Sobemoviruses encode serine-like 3C proteases (Pro) that participate in the processing and maturation of other virus-encoded proteins. Its cis and trans activity is mediated by the naturally unfolded virus-genome-linked protein (VPg). Here, we solved a full Pro–VPg 3D structure of ryegrass mottle virus (RGMoV) that demonstrates the structural changes in three different conformations due to VPg interaction with Pro. The overall fold change of Δ117Pro is typical for CLP and is very similar to the structure of SeMV Pro.

We crystallized and solved 3D crystal structures for two catalytically active forms of Δ117Pro: one in its VPg-free form, the second in its VPg-bound state with fused VPg at the C-terminal part (Δ117Pro-E/A-VPg), and one catalytically defective Δ117Procm form with S159/A mutation. First, in the absence of VPg, L87 shifted towards the VPg-binding pocket. In Δ117Pro chain A, it is rotated away from the catalytic triad H49, thereby disrupting the functionality of the catalytic triad since D92 is too far from H49 to ensure any proton transfer. There are several more conformational shifts unique only to Δ117Pro and that are not present in Δ117Procm and Δ117Pro-E/A-VPg. These are the partial unwinding of the βII barrel and subsequent movement of the bII and cII β-strands and the cII/dII loop, and the disordering of the eII/fII loop. While H173 and N183 did not change their positions significantly, H150 and T154 were noticeably shifted due to the movement of bII-cII strands. This shift could also render the Glu-binding site unsuitable for cleavage site recognition.

>AVANSIVSSVAPGKEPGSLVCIQAKDGKVIGMGARVHCGPATVLVTAGHVLKKGMIADLYLAKYSVSSKEGKRVLMDPTWKIEYGSLNKEADVISVQVPAAVWSRLGVTAARVRKPTVKVPVLAYGGEASGLLQSSQGFATPDGNMSVAHSCSTRPGWSGTPLYAGSDIVAIHRRWEDIGVKNLATNLSIFHANCESSE[2x]>[2x]MASVSSATFSGHGARSLLQFLRLVGQLKRVPRTGWVYRNVQRPESVSDHMYRMAVMAMVIKDDRLNKDRCVRLALVHDMAECIVGDIA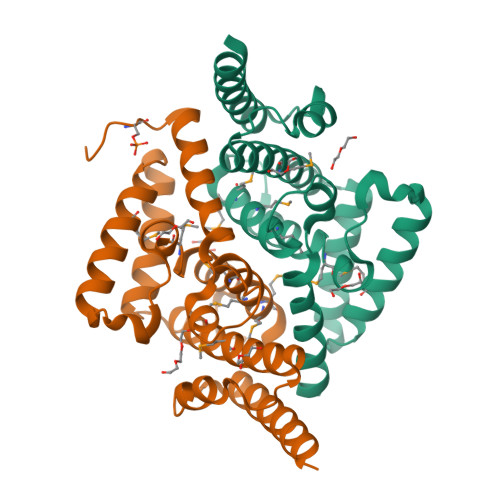PADNIPKEEKHRREEEAMKQITQLLPEDLRKELYELWEEYETQSSAEAKFVKQLAQCEMILQASEYEDLEHKPGRLQDFYDSTAGKFNHPEIVQLVSELEAERSTNIAAAASEPHS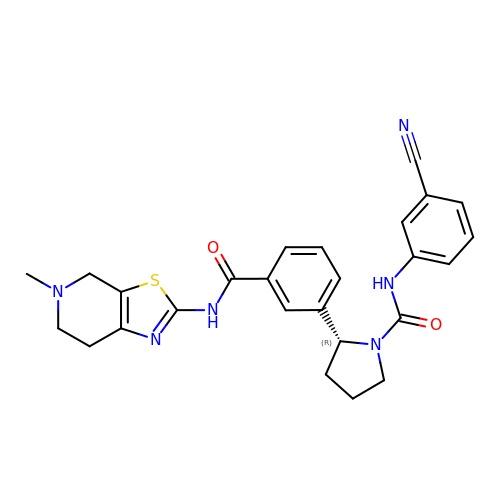(2R)-N-(3-cyanophenyl)-2-{3-[(5-methyl-4,5,6,7-tetrahydro[1,3]thiazolo[5,4-c]pyridin-2-yl)carbamoyl]phenyl}pyrrolidine-1-carboxamide | C26 H26 N6 O2 S | WSCPCHMPNPSKDY-JOCHJYFZSA-N> MYSDKVFDHFQNPRNVGKIEDADGVGTVGNPVCGDLMTIYIKVK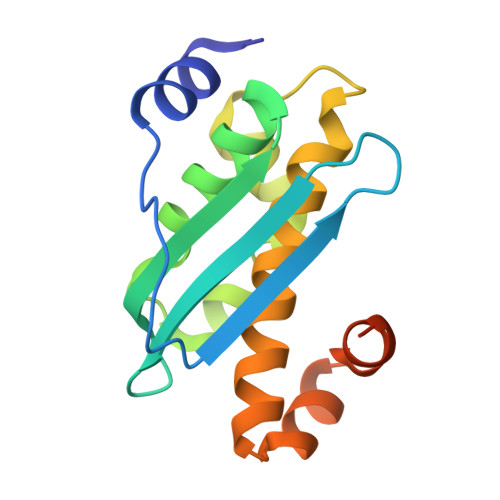DNRIEDIKFQTFGCAAAIATSSMATEMAKGKTIEEALKITRDAVAEALGGLPKQKMHCSNLAADALRRAIVDYFRKNGKIDKIKELGLEKELEKMEKGEMDDHGEYCEA> SNAEDTFKVGLIVPMTGGQASTGKQIDNAIKLYIKKHGDTVAGKKIEVILKDDAAIPDNTKRLAQELIVNDKVNVIAGFGITPAALAAAPLATQAKVPEIVMAAGTSIITERSPYIVRTSFTLAQSSIIIGDWAAKNGIKKVATLTSDYAPGNDALAFFKERFTAGGGEIVEEIKVPLANPDFAPFLQRMKDAKPDAMFV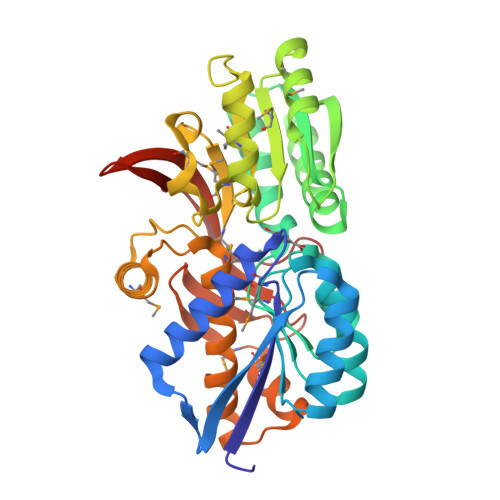FVPAGQGGNFMKQFAERGLDKSGIKVIGPGDVMDDDLLNSMGDAALGVVTAHMYSAAHPSAMNKEFVAAYKKEFGQRPGFMAVGGYDGIHLVFEALKKTGGKADGDSLIAAMKGMKWESPRGPISIDPETRDIVQNIYIRKVEKVDGELYNIEFAKFDAVKDPGKTKK> HMIFAKGH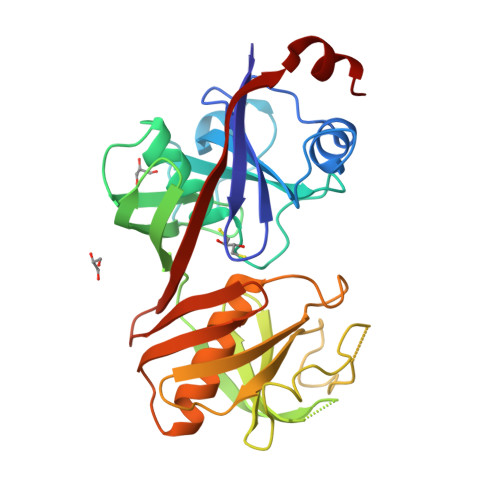GTQNDFVLLPDVDAELVLTAARVAALCDRRKGLGADGVLRVTTAGAAQAVGVLDSLPEGVRVTDWYMDYRNADGSAAQMCGNGVRVFAHYLRASGLEVRDEFVVGSLAGPRPVTCHHVEAAYADVSVDMGKANRLGAGEAVVGGRRFHGLAVDVGNPHLACVDSQLTVDGLAALDVGAPVSFDGAQFPDGVNVEVLTAPVDGAVWMRVHERGVGETRSCGTGTVAAAVAALAAVGSPTGTLTVHVPGGEVVVTVTDATSFLRGPSVLVARGDLADDWWNAMG>GPLGSKVDLFDFELPERLIAQVPLEQRDASRLMVLDKHTGELTDSSFKHIISFFNEGDCLVLNNTRVLPARLFGTKEDTGAKVELLLLKQETGDKWETL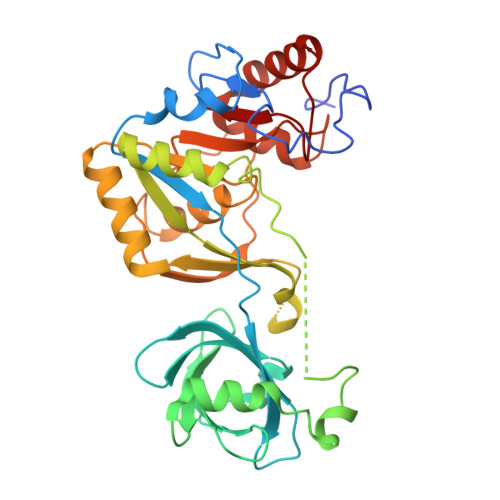AKPAKRVKKGTVVTFGDGRLKAICTEELEHGGRKMEFQYDGIFYEVLESLGEMPLPPYIKEQLDDKERYQTVYSKEIGSAAAPTAGLHFTEEILQQLKDKGVQIEFITLHVGLGTFRPVSADEVEEHNMHAEFYQMSEETAAALNKVRENGGRIISVGTTSTRTLETIAGEHDGQFKASSGWTSIFIYPGYEFKAIDGMITNFHLPKSSLIMLVSALAGRENILRAYNHAVEEEYRFFSFGDAMLII[2x]>[22x]MAMYINTNVPSLTAQRYLGETNNAVSKSLERLSSGLRINSASDDASGLAISEKLRGQISGLKRASLNAQDGISLLQTAEGGLQNIQDMLQRMRELAVQAGNGVYTTNDRAEIQKEVDQLKEEINRIASSTEFNTKKLLNGDSTALWSSDSSDLDVVIKSAVAEGNYNLNVTVDPGKNFVYKSDVM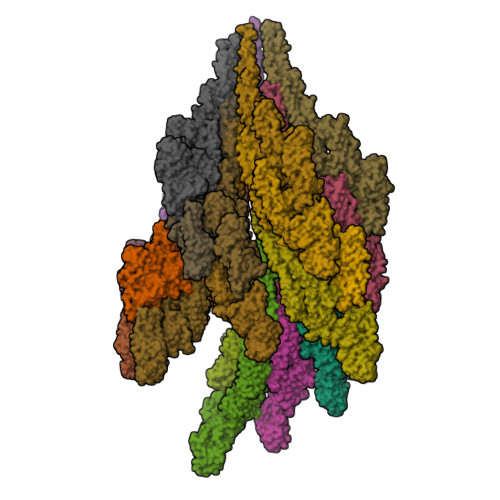TLNEDAIGAEIVTAGGDVNETNVGFVTDPNTLASTGTAYYTVDVTAGADTLSSVATMSVYRQAGSNFGSVATWTTGGTVADSGYLLIEAQENFTVSAGTTANYTFKATFVDAKTGEKSTYEIEGGDDGAGNLVFDLADMTGAGFSGEVSIAIGTDANMQSGDKILLSTTEAVDTSATSGGGTIAISGGPAGTTGAIISYGNNELTKVDNGDTTIDYNSVTVYHAALNVETGNLDVGNLTFNFREDTGTDTAYGSTTGGSFDLLVAGGGEAATSTTKLKDISRFTTDDGVNIFAAGPQELTIFGNGSSATIYLEGDDTVSEFETKLSSAILELGMGATAGTSDEAATVNSNLVNYVSTGDVTDSSNEALAGTFVIQTARLGDDSKLSFIGDQNLINALSLATIQEGENSETTIKVTDAHTGKFIGSDSVNDSTLRGVIQGVDVKIDSDVGVSISWNSTKKTMEFSATGESEDIKLHLVDNAMEMQIGANEGQTILANIPQVDTTSLGIDDILMVDQELAQESITKLDKALETVSGVRATIGAQINRLEYTMTGLDTTRENLTAAESRIRDLDIADEMAKFTKNQILAQSNISMLAQANSLPQMALSLLG>[4x]MKPTNYHLFDLFDFDTELLRDESLWKACKPTAVYEKDGDICVTVPFQKQLLANDMVADTAVPREEYTLIIRQYNIGITRLFLGFGEYELTDQSEMLQFSERIRRVPLSVEKQGGKWILFTQDGTKRAVINVEEPALDRWSELLPDPQETLDITLYPDGKREIRLAAYDHFSPPRYDGLP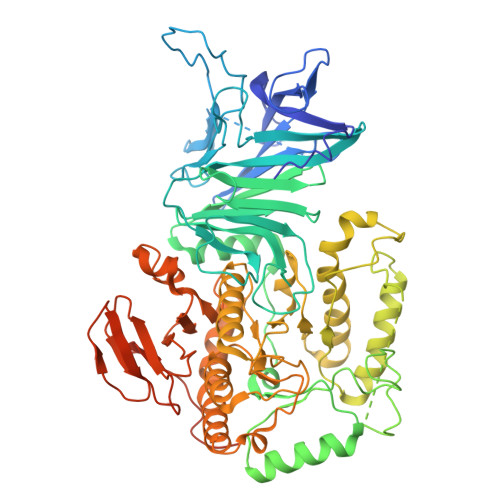IAFCKRTGKKERATLSFESRPDECFAGTGERFFKMDLSGQTLFLKNQDGQGVNNRRTYKNIPFYLSSRMYGTFYHTCAHSKLSLAGHSTRSVQFLSDQAMLDAFVIAGDTMEEILRGYRDLTGYPSMPPLWSFGVWMSRMTYFSADEVNEICDRMRAEHYPCDVIHLDTGWFRTDWLCEWKFNEERFPDPKGFIQRLKKNGYRVSLWQLPYVAEDAEQIEEAKANEYIAPLTKQQDTDGSNFSALDYAGTIDFTYPKATEWYKGLLKQLLDMGVTCIKTDFGENIHMDAVYKGMKPELLNNLYALLYQKAAYEITKEVTGDGIVWARAAWAGCQRYPLHWGGDSCSSWDGMAGSLKGGLHFGLSGFAFWSHDVPGFHTLPNFMNSIVAEDVYMRWTQFGVFTSHIRYHGTNKREPWHYPAIAPLVKKWWKLRYSLIPYIIEQSKLAVESGWPLLQALILHHPEDKLCWHIDDEYYFGNDFLVAPVMNSENRRDIYLPEGQWVNFFTGERLQGGRWLKEVYVPLEEMPVYVRENAVIPIYPEEVNCTDEMDLGKSIALRIDHNYKGFWTKHHHHHHLRVPRGS>[10x]HMAWDLKVKMLGGNDFLVSVTNSMTVSELKKQIAQKIGVPAFQQRLAHQTAVLQDGLTLSSLGLGPSSTVMLVVQNSSEPLSI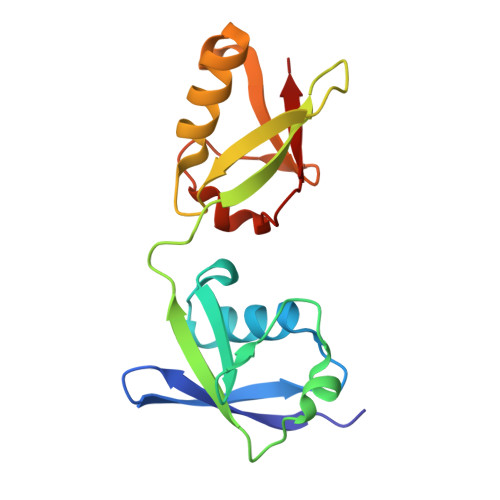LVRNERGHSNIYEVFLTQTVDTLKKKVSQREQVHEDQFWLSFEGRPMEDKELLGEYGLKPQCTVIKHL>GPMKTEMKDDFAKLEEQFDAKLGIFALDTGTNRTVAYRPDERFAFASTIKALTVGVLLQQKSIEDLNQRITYTRDDLVNYNPITEKHVDTGMTLKELADASLRYSDNAAQNLILKQIGGPESLKKELRKIGDEV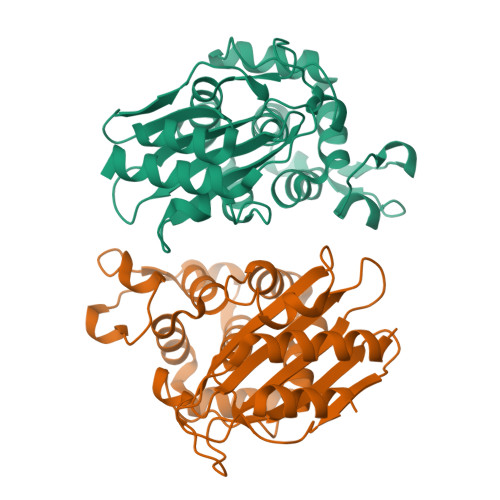TNPERFSPELNEVNPGETQDTSTARALVTSLRAFALEDKLPSEKRELLIDWMKRNTTGDALIRAGVPDGWEVADKTGAASYGTRNDIAIIWPPKGDPVVLAVLSSRDKKDAKYDDKLIAEATKVVMKALNMNGK[2x]The set of protein arginine methyltransferases (PRMTs) is a family of enzymes that catalyze the transfer of a methyl group from S-adenosyl-L-methionine (SAM) to the guanidino nitrogen of an arginyl residue to produce S-adenosyl-L-homo-cysteine (SAH) and methyl arginyl residues. TbPRMT6 is the homologue of HsPRMT6 in T. brucei with 31% amino acid identity. The overall monomeric structure of TbPRMT6 consists of three parts: a SAM-binding domain (residues 36–181, blue), a dimerization arm (residues 193–225, yellow), and a β-barrel domain (residues 182–192 and residues 230–368, green). The structures of TbPRMT6 highlight several structural features that are distinct from those found in previously characterized type I PRMTs, including four stretches of insertion, the absence of the β15 strand, and a unique dimerization arm.

To investigate the structural basis for the unique properties of TbPRMT6, we report the crystal structures of apo-TbPRMT6 and its complex with the methylation product SAH (SAH-TbPRMT6); these structures were refined at 2.20 Å and 2.35 Å, respectively. We primarily describe the structure of SAH-TbPRMT6 unless otherwise noted. The SAH molecule is enveloped in the deep pocket of the SAM-binding domain formed by the helixes αY, αZ, αA, αB, αC, and αD, and the strands β2, β3, and β4. (i) For the adenine ring moiety, the main-chain amide of V112 (helix αC) interacts with nitrogen N1, and the carboxyl group E113 (helix αC) and the hydroxyl group of S156 (helix αD) make a hydrogen-bond network with the amino group of the adenine ring of SAH. (ii) For the ribose moiety, the carboxyl group of E84 (strand β2) and the imidazole ring of H30 (helix αY) create hydrogen bonds with the two ribose hydroxyls. Upon SAH binding, the guanidine group of R39 moves inwards ∼3.9 Å, forming a hydrogen bond network with the carboxyl group of SAH, the backbone carbonyl of M33 of helix αY, and the carboxyl group of E142. The imidazole ring of H318 swings ∼5 Å to make a hydrogen bond with the carboxyl group of D36 of helix αY, and this hydrogen bonding interaction induces a 1.8-Å movement of the carboxyl group of D36. SAH binding appeared to fix the active site residues of TbPRMT6 in conformations that are favorable for substrate binding. Taken together, our structural observations and biochemical results suggest that SAH binding induces rearrangements of the active site that promote the substrate binding of TbPRMT6, thereby supporting an ordered mechanism in which a cofactor binds to the active site before the arginine substrate.

>[2x]MESGGFAEDYDPNSSLHHQYYESYSDLAVHRLMLEDAQRMSFYRKSIEQSASIEGKVVVDVGSGTGILSMWAARAGAKHVFSIEASSLSEFQIGVVEDNDLSTKITVLGDTVENIIAGGVANFVNRHKAKLGKCGVAVLLSEWMGFYLFHEGMLPSVIRARNFFQDVNAALGVLQPIEMIPERATVFVAPITCKPYYVQRYKNFWRDVDGLDFSRYGRIEYEVYLEQASPLVECLPPLCLLHEGLSLIELNLSTVQEEVLTSLHNTVHFDLKESAEFQQHAREAGSEGRVSVDGFTVWFDVSYGAHTLSTSPRSPSTHWKQTTILLPREARNEELVSFPVEGGELGVEMHISASDKTLRFYTIELELK>[4x]GMTGHIDPTKEVFAQFRANDREGPIHMLNLVRLRPRAAYPDG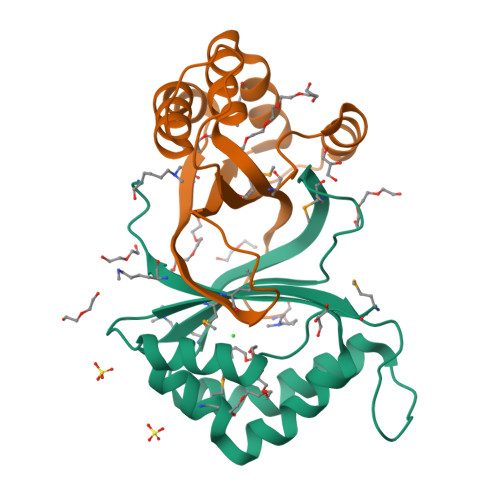RETTGAEAYAAYGRDSGPVSERLGGKVVWQGQFELMLIGPQDEHWDHVFIAEYPSVAAFVEMIRDPVYREAVKHRQAAVEDSRLIRLKPLKPGKGFGEIPT>[2x]ASEALTMIVNLLRSQRPLQEPTVEQMRAGLEAMAQMSPLPADVELTTVDAGGVPGAWVRVPESDPDRVVLYLHGGGYVIGSIRTHRDLAQRIARAARCRV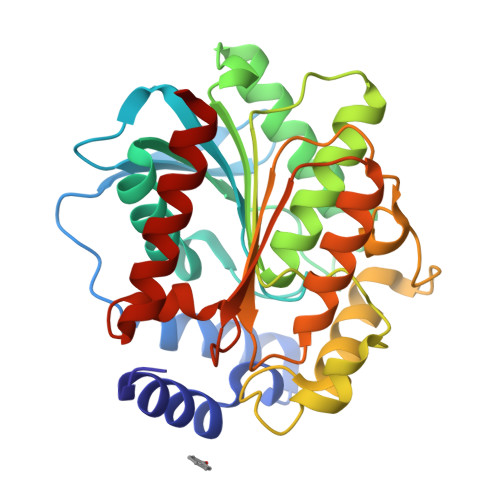LLIDYRLAPEHPHPAAVEDSTRAYRWLLETGSDPKRMAIAGDSAGGGLTVATLVALRDAGVPLPAAAVCLSPWVDLEGIGESMTTKAAVDPMVQREPLLRMASMYLAGQDPRTPLAAPLYADLRGLPPLLIQVGTAETLLDDSVRLAERARAAGVQVTLEPWEDMIHVWQAFAAMLPEGQQAIERIGEFLRQHWQ> MDSYFKAAVSDLDKLLD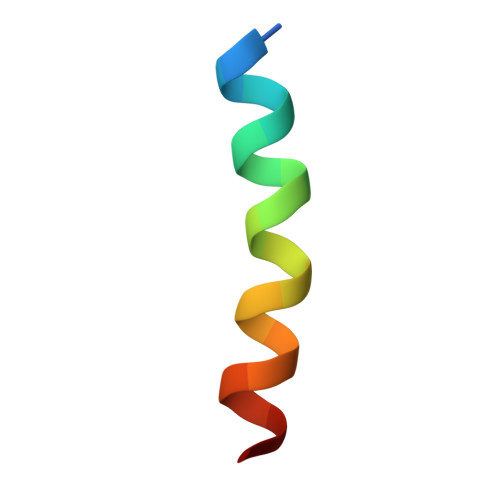DFEQN>[3x]SMNSHHHHHHGTACGLRSFTRQAAVVGGTDADEGEWPWQVSLHALGQGHICGASLISPNWLVSAAHCYIDDRGFRYSDPTQWTAFLGLHDQSQRSAPGVQERRLKRIISHPFFNDFTFDYDIALLELEKPAEYS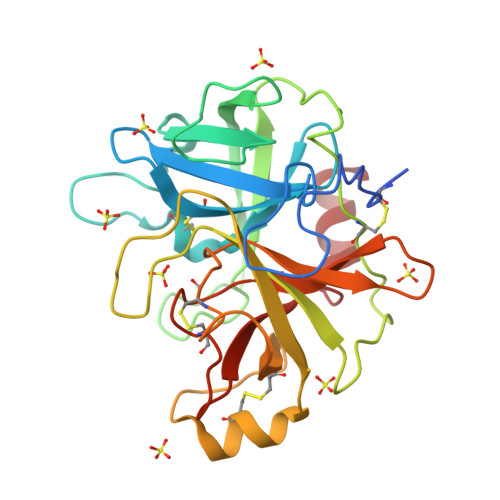SMVRPICLPDASHVFPAGKAIWVTGWGHTQYGGTGALILQKGEIRVIQQTTCENLLPQQITPRMMCVGFLSGGVDSCQGDAGGPLSSVEADGRIFQAGVVSWGDGCAQRNKPGVYTRLPLFRDWIKENTGV>MKKEPIKTSNPDNTESSDANEVEIENPTIAASGIVSVANTSDGRIEVFGVGGDNAVWRNGQTTHTGASWTGWSSLGGSVTSKPAAYLNSDGRLEVFVRGSDNALWHNWQTTPNASWSGWQSLGGALTSNPAVYINADGRLEVFARGLDNTLWHIWQTAPHSNPWSSWYSLGHVITSNPAVHINADGRLEVFARGADNALWHIWQTAPHSGYWSGWHSLGGVLSSDPVVARTVDGRLEVFVRAVDNALWHIWQTAPNSSQWSNWASLGGTITSAPAVIKYFDNRLVVFARAIDNALWHIWQNDTHSGSWSNWGSLGGGLSSGPDVVENANGYIEVFVRATDNALWNIKRTSPSSWSSWASLGGTLID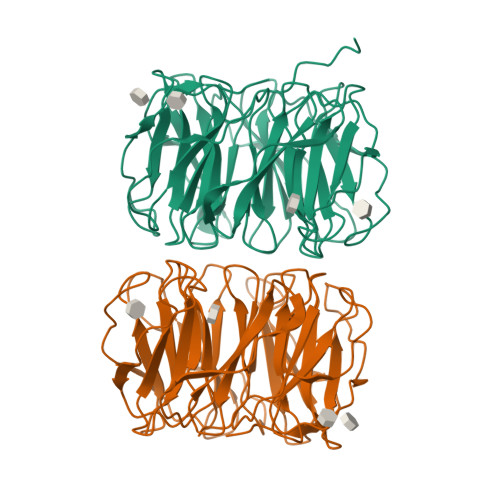ASAIK[4x]Species D (HAdV-D) are the most diverse species and cause both gastrointestinal tract infections and epidemic keratoconjunctivitis (EKC). Each protein forms key interactions to promote cell infection, with the terminal domain of the fiber, the fiber knob protein, interacting with the viruses’ primary cell entry receptor. The adenovirus fiber knob protein is known to have a highly conserved trimeric structure. Sialic acid (SA) usage has been proposed as a major mechanism of cell infection for EKC causing HAdV-D. Here, we provide apo state crystal structures for fiber knob proteins of 7 previously undetermined HAdV-D, and provide crystal structures of HAdV-D25, HAdV-D29 and HAdV-D53 knob proteins bound to SA.

We performed X-ray crystallography to generate structures of species D human adenovirus fiber knob proteins HAdV-D15, D24, D29, D30, D32 and D53 in their apo states. These structures show the expected trimeric form, all viewed down towards the apical domain of the fiber knob proteins ([Fig fig1]). HAdV-D15, D24 and D32 were crystallised in only their apo states, whereas HAdV-D25, D29, D30 and D53 crystals were also soaked with sialic acid. The observed space groups were monoclinic (P2_1_ P2 or C2), orthorhombic (P2_1_2_1_2_1_), trigonal (H3 – R3 in hexagonal axes) or cubic (P23). However, there were varying numbers of monomers or trimers in each asymmetric unit, presenting a diverse picture of the fiber knob interactions. In this article we present seven novel structures of apo state fiber-knob proteins of species D adenoviruses ([Fig fig1]). These provide a good basis from which to conduct structural analyses.

>[6x]VGNKNNDKLTLWTTPDPSPNCKVSEEKDSKLTLVLTKCGSQILASVSLLVVKGKFANINNETNPGEDYKKFSVKLLFDANGKLLTGSSLDGNYWNYKNKDSVIGSPYENAVPFMPNSTAYPKIINNGTANPEDKKSAAKKTIVTNVYLGGDAGQPVATTVSFNKETESNCVYSITFDFAWNKTYKNVPFDSSSLTFSYIAQDAEDKNE>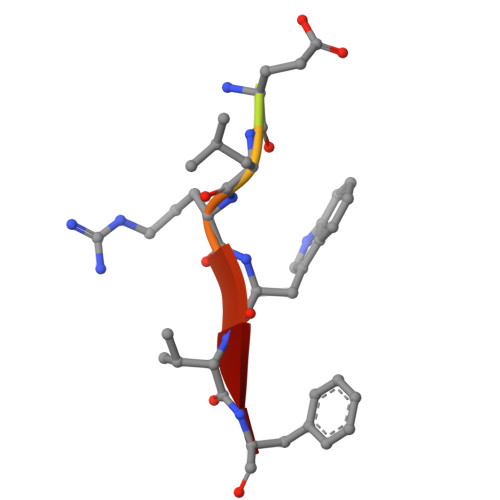 SVRDELRWVF>[2x]GPNANPIPEHFFAPYIDMSLSVHKPLVEYAKLTGTKYFTLAFILYSSVYNGPAWAGSIPLEKFVDEVRELREIGGEVIIAFGGAVGPYLCQQASTPEQLAEWYIKVIDTYNATYLDFDIAAGIDADKLADALLIVQRERPWVKFSFTLPSDPGIGLAGGYGIIETMAKKGVRV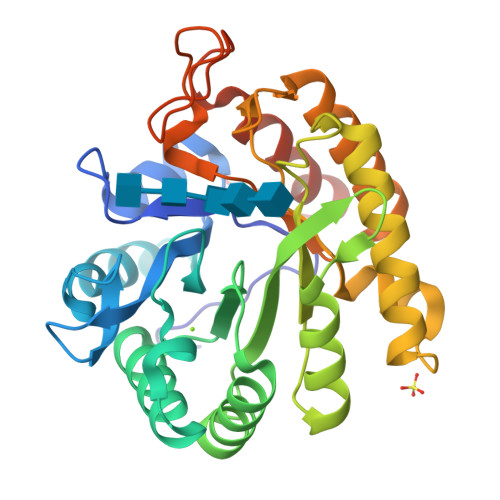DRVNPMTMDYYWTPSNAENAIKVAENVFRQLKQIYPEKSDEEIWKMIGLTPMIGVNDDKSVFTLEDAQQLVDWAIQHKIGSLAFWSVDRDHPGPTGEVSPLHRGTNDPDWAFSHVFVKFMEAFGYTFSAQTSEASVPT3-bromo dicyclotyrosine | C18 H17 Br N2 O4 | 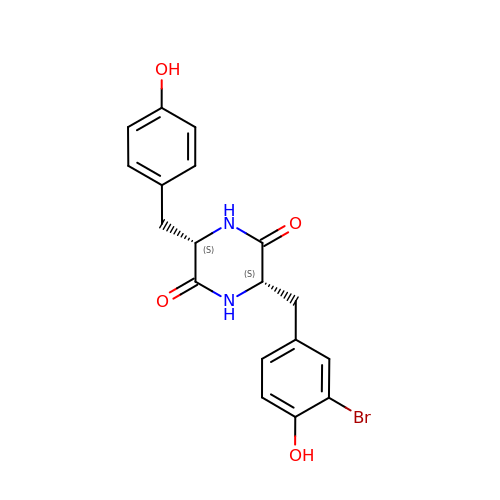UHZMUUVMCUUKRQ-GJZGRUSLSA-N> MKHTLPDLPFDYADLEPVISHEIMQLHHQKQHATYVNNLNQIEEKLHEAVSKGNLKEAIALQPALKFNGGGHINHSIFWTNLA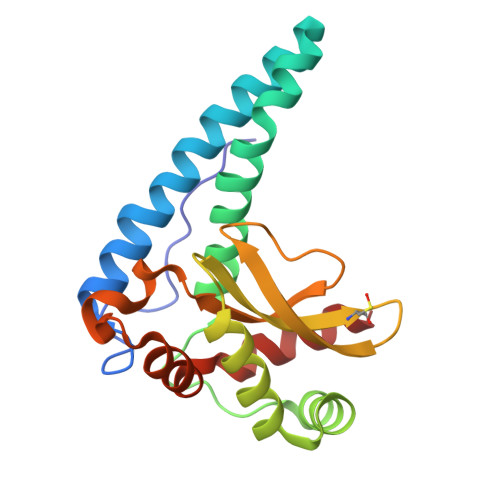KDGGEPSKELMDTIKRDFGSLDNLQKRLSDITIAVQGSGWGWLGYCKKDKILKIATCANQDPLEGMVPLFGIDVWEHAYYLQYKNVRPDYVHAIWKIANWKNISERFANARQ> GUGGUCUG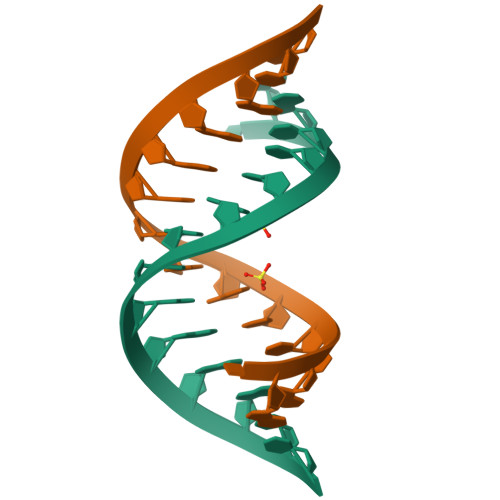AUGAGGCC> NRKLNFGQAVEALKKGKRVARQGWNGKGMFIFQRPGDELSKTFLPNVKSLPDAVKKFLMDQDRDIEFTPYFCMYSASGDIVNGWLASQTDMQ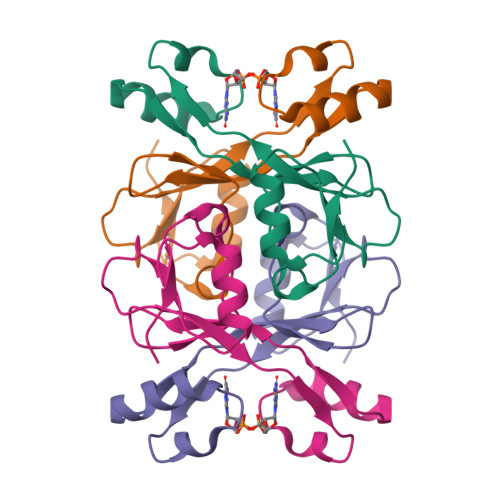AEDWFVLED>[2x]MIIVYTTFPDWESAEKVVKTLLK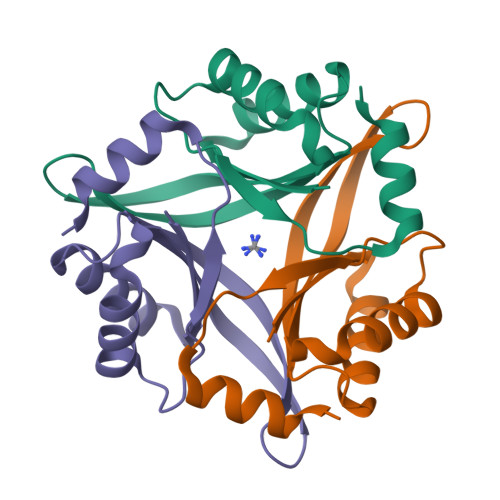ERLIACANLREHRAFYWWEGKIEEDKEVGAILKTREDLWEELKERIKELHPYDVPAIIRIDVDDVNEDYLKWLIEETKK>[5x]NAMIIRPEQHWFLRLFDWHGSVL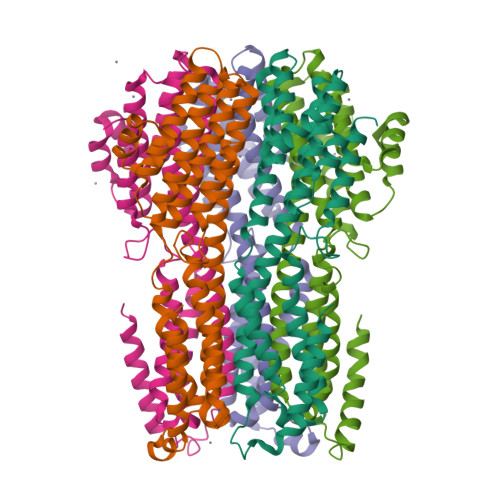SKIIFRLLLNVLMSIIAIISYQWYEQLGIHLTVAPFSLLGIAIAIFLGFRNSASYSRFVEARNLWGTVLIAERTLVRQLRNILPAEHDAHRRIVSYLVAFSWSLKHQLRKTDPTADLRRLLPEERVTEILASSMPTNRILLLAGNEIGQLREAGKLSDTTYGLMDNKLDELAHVLGGCERLATTPVPFAYTLILQRTVYLFCTLLPFALVGDLHYMTPFVSVFISYTFLSWDSLAEELEDPFGTAANDLPLNAMCNTIERNLLDMTGQHPLPE>[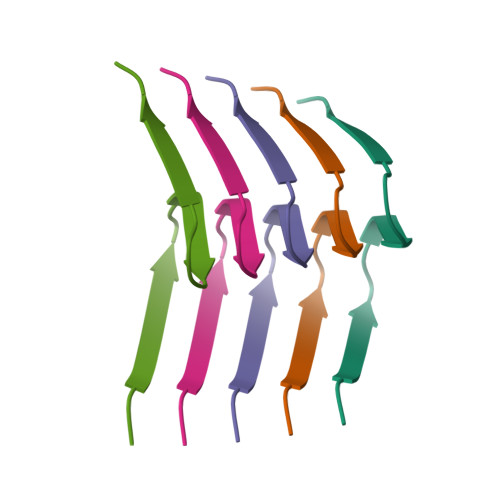5x]HMPSLHNIPVPETNYLGNTPTMPFSSLPPTDESIKYTIYNSTGIQIGAYNYMEIGGTSSSLLDSTNTNFKEEPAAKYQAIFDNTTSLT> GNSKSGALSKEILEELQLNTKFTEEELSSWYQSFLKECPSGRITRQEFQTIYSKFFPEADPKAYAQHVFRSFDANSDGTLDFKEYVIALHMTSAGK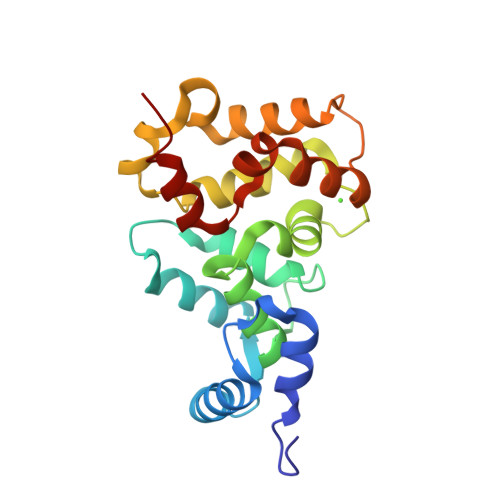TNQKLEWAFSLYDVDGNGTISKNEVLEIVTAIFKMISPEDTKHLPEDENTPEKRAEKIWGFFGKKDDDKLTEKEFIEGTLANKEILRLIQFEPQKVKEKLKEKKL> GAMGSMRLLVSCVDSGSIKEVLCNIGTDTSVQSALQPFHVAPHLAEGLKAYVDRMWVISEDEAILARNSGVVELVKISKHLKENEALQVDPKGESKNEKSLSDDLPKFDISEFEITSSVSDLFDDAKLESLSSKSVKRTKLVDGFVTLCPIKKDSSNNTFVAATKSGLLHIIKKGEDKKLIKLASLGLKAPVEFLQLYDLEDTDTDKYIFAYGGEENLIKLVEIDSSFQSLKQIWEAKNVKNDRLDMRVPVWPMALRFLEPSPGKTEKGKLNYQFAAITRWSH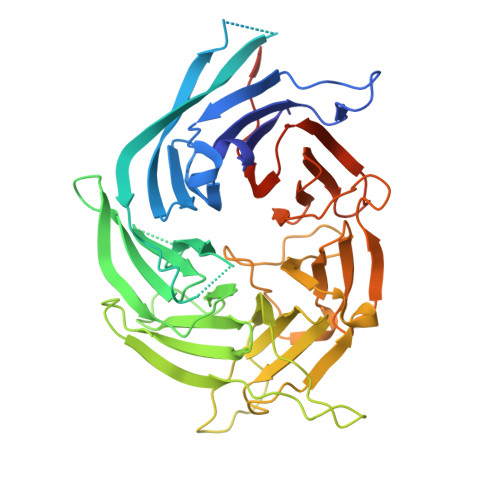LTKYSTQHGRKPFAQIDLLPNREPLSQMEVFDAKGENVVSSLGNFQSETFNELNVITTDYKKNVFKFDGNGRMLGKVGRDDITGSSTYIHVHDGKYLLQGGLDRYVRIFDIKTNKMLVKVYVGSRINFIVMLDDVEIEMPLSPSAKAAKGKQKRKV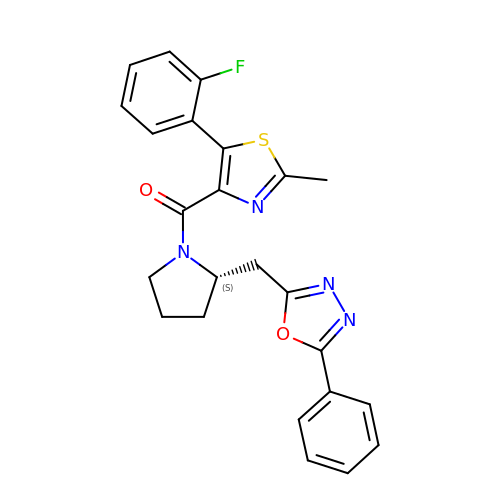[5-(2-fluorophenyl)-2-methyl-1,3-thiazol-4-yl]{(2S)-2-[(5-phenyl-1,3,4-oxadiazol-2-yl)methyl]pyrrolidin-1-yl}methanone | C24 H21 F N4 O2 S | HYBZWVLPALMACV-KRWDZBQOSA-N> GPGDQRFGDLVFRQLAPNVWQH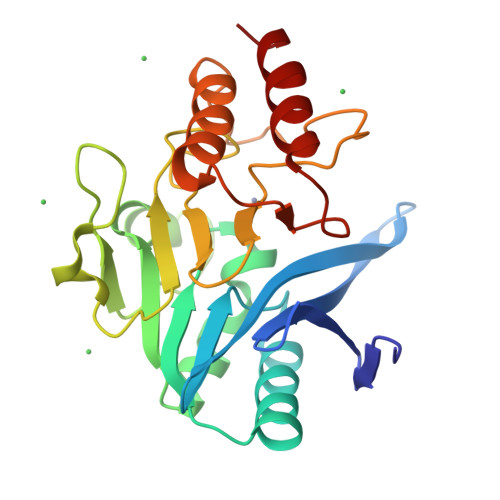TSYLDMPGFGAVASNGLIVRDGGRVLVVDTAWTNDQTAQILNWIKQEINLPVALAVVTHAHQDKMGGMDALHAAGIATYANALSNQLAPQEGMVAAQHSLTFAANGWVEPATAPNFGPLKVFYPGPGHTSDNITVGIDGTDIAFGGCLIKDSKAKSLGNLGDADTEHYAASARAFGAAFPKASMIVMSHSAPDSRAAITHTARMADKLR>MAPTWFYNTTNSEKLRELQHVLGGSAKLGYLTAKVTEILDVDLETVIRAKAIAAYRAVRVPVIVEHGALCIDALNGLPGALVKPFWESLDTRLCEVIPAGQRTARARGALCYCDGRERHVLIEETEGEIAPSARGTGGFHWDPIFIPKGQTRTFAEMSLDEKLSFSPLGRLHTRLRTELGL[8x];>[8x]MTTLTLSEAAPLLKKEFREGRLIPFLGAGFSKPLKLPDGSQLIASLAKTLGFEPELFDMHGRFEQLAEFFAISAPNRLQRLVYEMSLSFDSAEAEALREKSPMHRALAALDWRTIYTTAYDKHVEGALRDAGKQAAVLAS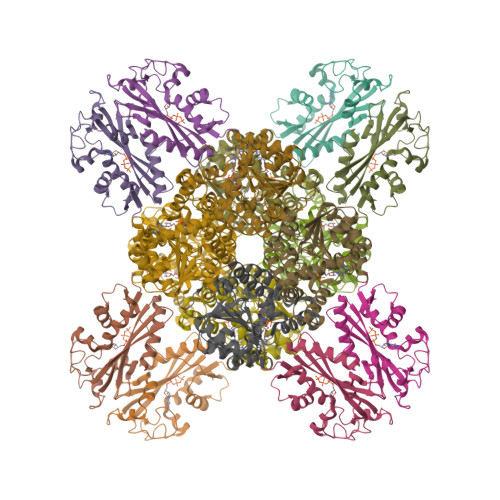FADFQGPRARDVCEVIKFAGTLDQPDTIVLTESSYFQRMALDAPPDQRLRADLLANSFLFIGYSFSDTNIRYIWYRMNQLREQSQLGVKHSQARRCFFATHGAGLVQPDILQQWNIDVIQLDPTDKSASVARLLESIA> MRGSHHHHHHGSASYEYTSKEELKKTIHAAYLLLDGEFEGIDDSQKDNRVPEVDRTPAEIIAYQLGWLHLVMGWDRDELAGKPVIMPAPGYKWNQLGGLYQSFYAAYADLSLTELRRLFRDTERQWLDWIDTLSEEDLFTQSVRKWTGDKPNWPMARWIHINSAAPFKTFRAKIRKWKKHQRQA

The precursor PdDfsB is cleaved by subtilisin to yield biologically active Slf, and the chemical gradients of both proteins between two growing colonies could be accurately modelled. However, remarkably, the dfsB gene is widely distributed across Gram-positive and to some extent Gram-negative bacterial kingdoms (PFAM entry DUF1706). PdDfsB adopts a four-helical bundle core structure that belongs to the DinB structural superfamily. The most strongly conserved region of PdDfsB is the C-terminal helix, which is present within the mature Slf sequence.

A 12-kDa polypeptide was shown to be localised exclusively to this region and is derived from a precursor protein termed DfsB (PdDfsB). To help understand structural changes upon DfsB/Slf conversion, we crystallised recombinant, His-tagged PdDfsB and solved its atomic structure using X-ray crystallography. PdDfsB does not follow this pattern: it is a monomer and lacks the conserved residues responsible for coordinating metal ions. Also uniquely, the C-terminal helix of PdDfsB contains a conserved proline that introduces a kink in the helix. Finally, PdDfsB displays a strong positively charge patch that is, again, absent from other DinB family members. Coupled with the fact that PdDfsB is apparently secreted and processed extracellularly, our structural data suggest that it is not an enzyme. The processing site for subtilisin is highly solvent exposed and found within a flexible loop. Cleavage by subtilisin results in one of the central α-helices being removed, which would force the remaining polypeptide to collapse to a new state, or oligomerise, or bind other hydrophobic surfaces such as a lipid bilayer. The remaining sequence of Slf is shown in Fig. 1e, and it includes many conserved positive charges and aromatic residues. The pattern of conserved positive charge and aromatic positions is reminiscent of cationic antimicrobial peptides, which damage cell membranes.>[6x]MTQFNITWEEQLQALSKLDGLHHPHKLEDISVHWVFNPVDISVFVTCATMSSHNTHYTFKPQSSPDDAMVREYVLSRIIADNLKYVDNLYLAAGAVICGNDEYISDGNVVGIHIADGVGGNKLILPVIEFMPGVHVDDISDKLIKSSSYQGIFKTDNLEEFEFLVDKKNANNVKELILAYTDYFANKLAFKDPAEPAVEMYQFIDRTEVYFSFEGCHPDVEEVLFTIKIVRYNQPLNSTAMQVFLKNPLLSHIRTVVRQDLPAKFVGGVLFNFKGHHHHHH;>[6x]ERPRRRSRGQRRRSNRRERQ

By performing a screen based on affinity purification and mass spectrometry, we observed that a previously uncharacterised phage protein specifically binds to two RNA binding sites within the CTH of RNase E, and by doing so efficiently inhibits the RNA binding and degradation activity of the degradosome assembly. We have determined the structure of this protein (termed Dip, ‘degradosome interacting protein’) by X-ray crystallography and show that it forms an open-clamp like homo-dimeric structure, and binding of Dip to RNA binding regions within RNase E is characterized functionally and structurally. As with the 756–775 binding site, 9S rRNA can be competitively displaced from the 583–636 fragment by Dip, and the addition of a 4-fold excess of Dip is able to completely remove the bound RNA from the RNase E fragment. These results demonstrate that Dip targets both RNA binding sites in the C-terminal half of the RNA degradosome, and consequently blocks the binding of RNA to the RNase E subunit.

To further study the interaction between Dip and RNase E, modelling experiments were performed to predict the binding surface for one of the Dip binding peptides of P. aeruginosa RNase E (residues 756–775). Secondary structure prediction of this RNase E peptide in isolation suggested a high propensity towards a helical conformation. Therefore, this helical form of the peptide was used in a docking experiment intended to scan the complete surface of Dip with the DOT docking program. The best energetically ranked complexes show binding of the peptide to a negatively charged patch on the outer surface of the Dip-dimer. To verify the in-silico docking results Dip was co-crystallized with the 756–775 peptide of P. aeruginosa RNase E. Hexagonal crystals of Dip were obtained containing an apparent ring-like hexamer of Dip formed through crystallographic symmetry. Discontinuous density was observed on the surface of Dip in the DOT docking predicted acidic pocket. Processing the X-ray diffraction data in the lower symmetry P1 space group visibly improved the density for the RNase E peptide, and we were able to cautiously model eight amino acids of the peptide into this density. The model of Dip bound to the short RNase E recognition peptide (Dip:RNaseE756-775) indicated significant contacts are made between residues Asp 137, Asp138, Glu 214 and Glu 222 of Dip and the RNase E peptide. A double mutation of Glu 214 and Glu 222 to alanine was sufficient to completely abolish the interaction with both Dip binding sites on RNase E when assessed by an electrophoretic mobility shift assay. There were no other significant alterations to the local or overall structure of Dip (data not shown). These data show that the acidic patch on the outer surface of Dip is crucial for the interaction with RNase E, and both of the RNA binding segments of RNase E engage Dip via this region.>[2x]MAVPETRPNHTIYINNLNEKIKKDELKKSL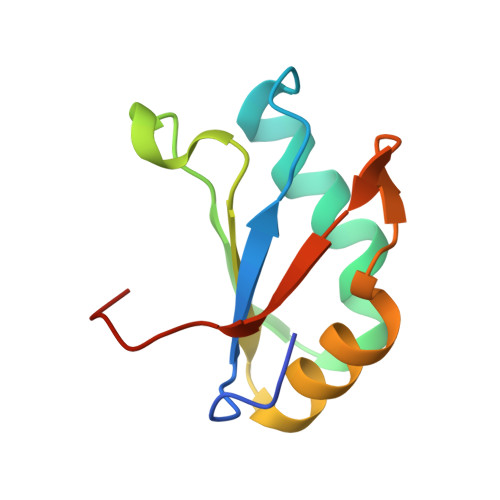YAIFSQFGQILDILVSRSLKMRGQAFVIFKEVSSATNALRSMQGFPFYDKPMRIQYAKTDSDIIA>GSALEKVPVEEYLVHALQGSVSSGQAHSLASLAKTWSSGSAKLQRLGPETEDNEGVLLTEKLKPVDYEYREEVHWMTHQPRVGRGSFGEVHRMKDKQTGFQCAVKKVRLEVFRVEELVACAGLSSPRIVPLYGAVREGPWVNIFMELLEGGSLGQLIKQMGCLPEDRALYYLGQALEGLEYLHTRRILHGDVKADNVLLSSDGSRAALCDFGHALCLQPDGLGKSLLTGDYIPGTETHMAPEVVMGKPCDAKVDIWSSCCMM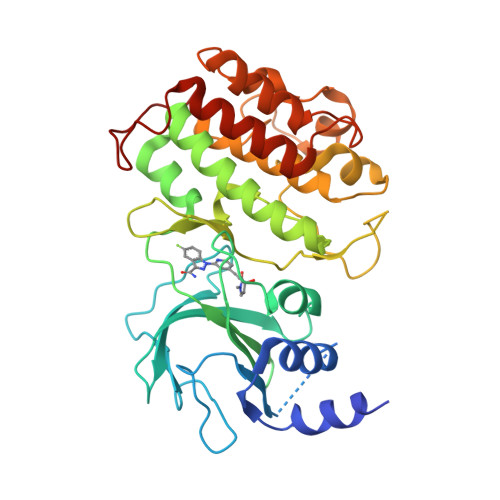LHMLNGCHPWTQYFRGPLCLKIASEPPPIREIPPSCAPLTAQAIQEGLRKEPVHRASAMELRRKVGKALQEVGGLKSPWKGEYKEPR[2x]>[2x]FQGM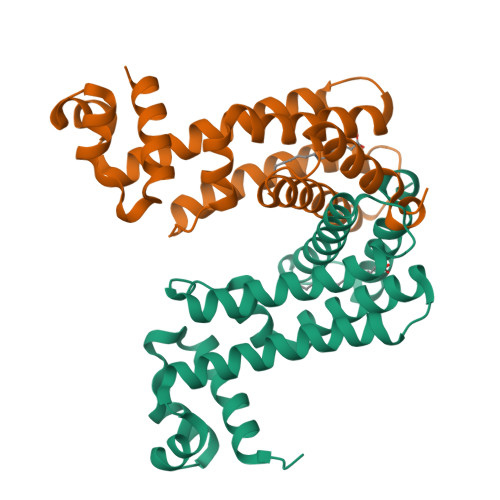LPRDERRGQLLVVASDVFVDRGYHAAGMDEIADRAGVSKPVLYQHFSSKLELYLAVLHRHVENLVSGVHQALSTTTDNRQRLHVAVQAFFDFIEHDSQGYRLIFENDFVTEPEVAAQVRVATESCIDAVFALISADSGLDPHRARMIAVGLVGMSVDCARYWLDADKPISKSDAVEGTVQFAWGGLSHVPL ethyl 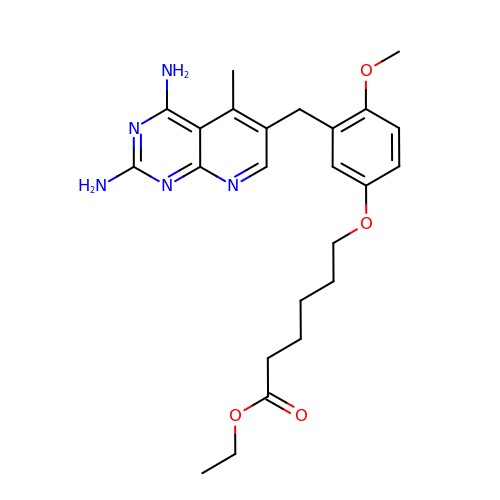6-{3-[(2,4-diamino-5-methylpyrido[2,3-d]pyrimidin-6-yl)methyl]-4-methoxyphenoxy}hexanoate | C24 H31 N5 O4 | FGBRLIYQKRWOSO-UHFFFAOYSA-N> MDPQTLITKANKVSYYGNPTSKESWRYDWYQPSKVSSNVQQPQQQLGDMENNLEKYPFRYKTWLRNQEDEKNLQRESCEDILDLKEFDRRILKKSLMTSHTKGDTSKATGAPSANQGDEALSVDDIRGAVGNSEAIPGLSAGVNNDNTKE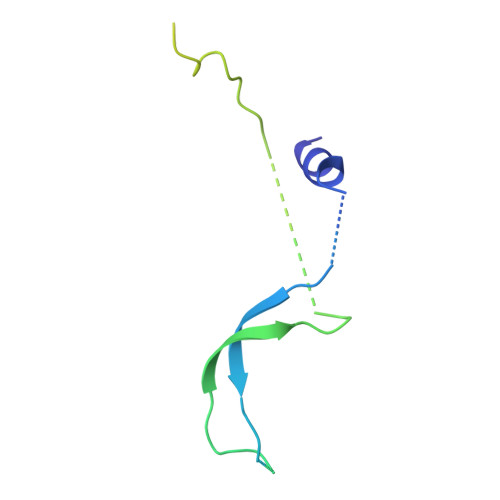SKDVKMN>[2x]DFGLDCDEHSTESR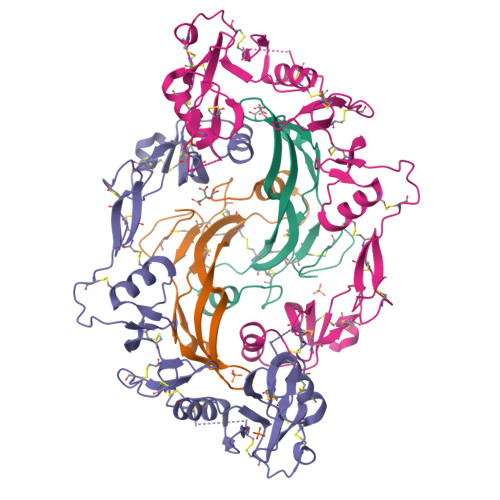CCRYPLTVDFEAFGWDWIIAPKRYKANYCSGECEFVFLQKYPHTHLVHQANPRGSAGPCCTPTKMSPINMLYFNGKEQIIYGKIPAMVVDRCGCS;>[2x]GNCWLRQAKNGRCQVLYKTELSKEECCSTGRLSTSWTEEDVNDNTLFKWMIFNGGAPNCIPCKETCENVDCGPGKKCRMNKKNKPRCVCAPDCSNITWKGPVCGLDGKTYRNECALLKARCKEQPELEVQYQGRCKKTCRDVFCPGSSTCVVDQTNNAYCVTCNRICPEPASSEQYLCGNDGVTYSSACHLRKATCLLGRSIGLAYEGKCIKAKSCEDIQCTGGKKCLWDFKVGRGRCSLCDELCPDSKSDEPVCASDNATYASECAMKEAACSSGVLLEVKHSGSCN>MGSSHHHHHHSQDPMACKIENIKYKGKEVESKLGSQLIDIFNDLDRAKEEYDKLSSPEFIAKFGDWINDEVERNVNEDGEPLLIQDVRQDSSKHYFFILKNGERFDLLTREFDSFTSPDLTNEIKEITDQLSYYIYNKHFSSDFEQVEGAKLNIQNEISQFVKEGKAPVQAAYNKLQDPDIKDLLDYYDNIEKHSDEFESEIVKFFSEKKLIIKDAELEDVTQEGLNEGLQGGDLVQAFEKNSKDNATANVKLMLSFLPKIDNLTGEPALGDYLNKPVFRSFDSIHSELLEVLSDITTLHVQGEVLDVFSSMYNKIKELADFKKSFKPLLEILDTIDEQKKTEFVQAFYLSKINFYTTTIETLETEDQNNTLTTFKVQNVSNANNPISSKLTEYYTNFKYKILPGGKLNKGKLKDLQSTVTSLLEKTRKENNPKYKSDSDFYEVFEEGVVELMQVFEDLGVDSITFEAMDIFLKQFRFDLPENNAYKIMYQQYQGKLTNLNNLLKDIQSNKINPYKINPFKNYSNLIFNSLAEAENYFIENNNESTIFSNGKTYWNFARPSYISNRINTFKNNPGVLRQLLNTSYGQSSLWAKHLLGEEKNVTGDFVLAGNARESASENRLKSLELSIFNSLQEKDKGAEGNDNGSISIVDQLADKLNKVLRGGTKNGTSIYSTVTPGDKSTLHEIKIDHFIPETISSFSNGTMIFNDKIVNAFTDHFVSEVNRMKEAYQELETLPESKRVVHYHTDARGNVMKDGKLAGNAFKSGHILSELSFDQITQDDNEMLKLYNEDGSPINPKGAVSNEQKILIKQTINKVLNQRIKENIRYFKDQGLVIDTVNKDGNKGFHFHGLDKSIMSEYTDDIQLTEFDISHVVSDFTLNSILASIEYTKLFTGDPANYKNMVDFFKRVPATYTNGTNLRLGLEANDHLFDVAVLENIVKPSAYLKEIGESLKLSDLSEAEKKYILEAYEDVNQTDAQAWITPKRWAFLISRTGKWNSKYQSVYNKILKSESLDASEMKLAAQPLKGVYFGLVNNTPTYLKYSQAVLLPQLVAGTQLQSLADAMNKQDIGESIVLDGVKVGATTPNIVTDENGDILKSISLNPLTLSNADWKLQQDLPVKTIKPTLLGSQIQKNIYSSLTDEATYTIENEAFNGSGMFQAINDTVSAMSNLSIAGLSSELGKDSEGKIDKRKLYDMLEREMLDKGSAINLLKSIQKNLPIEAMPGIKDKLYNIVFSKINSAAVKLKTNGGSFIQLSNFGLDKQTADAKGITWLVEPSDLKPPVIEKDADGKNYIRPGQIFMSHVQIAKLVPDYAKMDSKTLSSMIDPKALRAIGYRIPNQGQSSNDPLQIVGILPEAMGDTIVAYTEIPTKTGSDFDID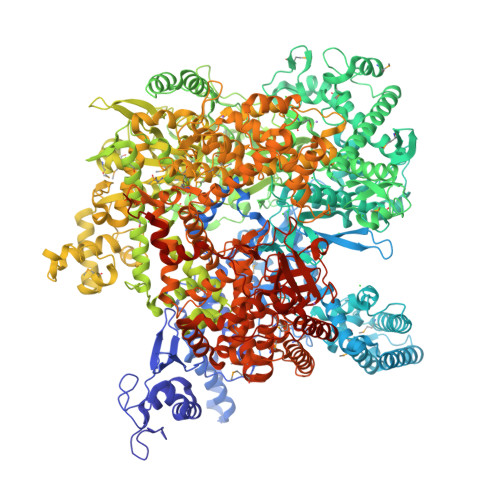KMYVMLPNFKVEHTKKSFKLAKDYIAQNEITVEEMYDELEDHGFNIDDIANGEEVTESAITEAFIKNHILNSNSELEYHNDFVKQHNIDAVNKIDFLGYSEELHKNKSEQLQNRLFDLYWAVLTNEKTYGDLITPIDFPHVKDEIKRVFGDNSKQTGENLKFHDPLYQLKLKFTYAGGKSGVGITANMLVDHNRSKGIDMQFNQYNLGVGHTQNGNTVFDKEYSEELNGTRFKIKDTISAFLNAFVDNAKDPYINDGNFNTYTSSVAFMLIRAGVHPDWIISFIGQPVLRELADFTQRYESKIIPKEDVGKSSFDIIVEKYETINQESYKDAESRAFSLDTLQESIEVGVHGIDLDVLKTFKGFQEQAKRLNESVQLSRFDTNGSGKNILDLIILKNKIKNLYVSEQTQQKGSMMNHFKKYHNNGKITSLGTQVKNTLLFTDDILNNNPSLFLLGSKPIQDLVNSISNNLVDSRGGSRGLLTNEDVGKLFYKEVYKYIMADFAPFKVGDPMAYIKDTIFDLVNYKTEDKQYDSSNFFIENMTVYENSFGITNKNKSVDFQDRLYRSAYDLMMENPELANKMFISSFLMNGFENKLIDIKEYIPYQWFLENDIRSFIESKNTGLKDSSESLRSFEEQFIKNNSDSNILAPKVSQSVIKSIKGIKSKHVFELPINDKTKRYILGATETKEEVLPNYVKVGSDLYRLKAYREKSGVYVRTNKLGFEDPKSFLSIKEYKFGTRTGGNFTGELTKQELVYTNQWVNENITLANGYISADSRTVDNPADKILEQNSLENILFSQNNVVSSDENDITKQECK[2x]>[2x]SMDLLVPKLTASVTDGAVGVTVDAPVSVTAADGVLAAVTMVNDNGRPVAGRLSPDGLRWSTTEQLGYNRRYTL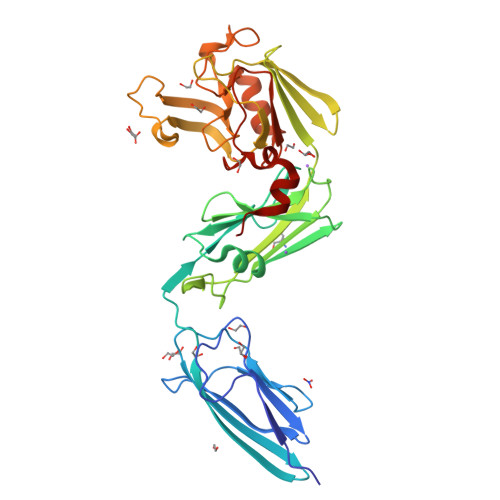NATALGLGGAATRQLTFQTSSPAHLTMPYVMPGDGEVVGVGEPVAIRFDENIADRGAAEKAIKITTNPPVEGAFYWLNNREVRWRPEHFWKPGTAVDVAVNTYGVDLGEGMFGEDNVQTHFTIGDEVIATADDNTKILTVRVNGEVVKSMPTSMGKDSTPTANGIYIVGSRYKHIIMDSSTYGVPVNSPNGYRTDVDWATQISYSGVFVHSAPWSVGAQGHTNTSHGCLNVSPSNAQWFYDHVKRGDIVEVVNTVGGTLPGIDGLGDWNIPWDQWRAGNAKA>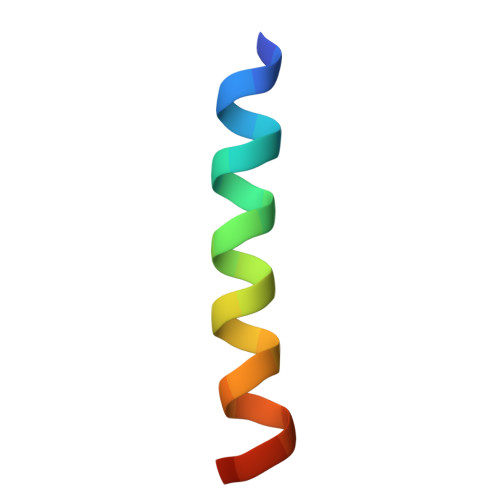 DDQQLDHNFKQMEEHLALMVEGNE> TLSILVAHDLQRVIGFENQLPWHLPNDLKHVKKLSTGHTLVMGRKTFESIGKPLPNRRNVVLTSDTSFNVEGVDVIHSIEDIYQLPGHVFIFGGQTLYEEMIDKVDDMYITVI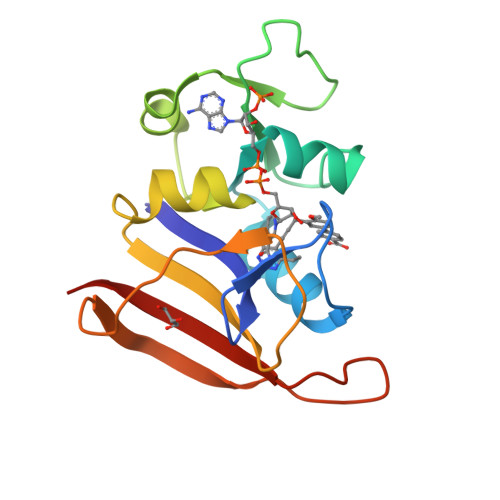EGKFRGDTFFPPYTFEDWEVASSVEGKLDEKNTIPHTFLHLIRKLEH>[2x]EAPYASLTEIEHLVQSVCKS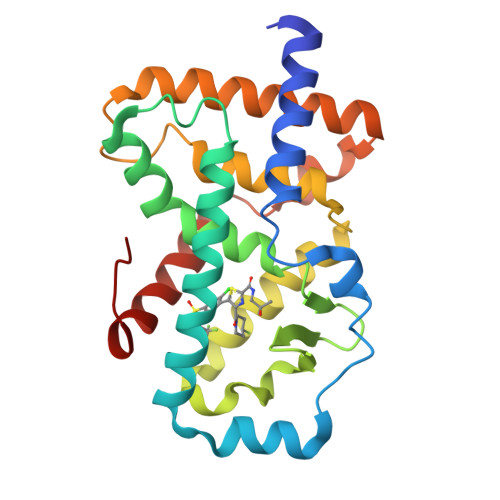YRETCQLRLEDLLRQRSNIFSREEVTGYQRKSMWEMWERCAHHLTEAIQYVVEFAKRLSGFMELCQNDQIVLLKAGAMEVVLVRMCRAYNADNRTVFFEGKYGGMELFRALGCSELISSIFDFSHSLSALHFSEDEIALYTALVLINAHRPGLQEKRKVEQLQYNLELAFHHHLCKTHRQSILAKLPPKGKLRSLCSQHVERLQIFQHLHPI1'-(1H-indazol-7-ylcarbonyl)-6-methylspiro[chromene-2,4'-piperidin]-4(3H)-one 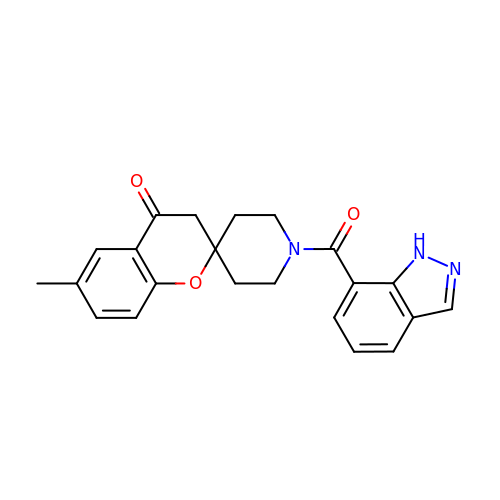| C22 H21 N3 O3 | IKCMGTBANLMNNP-UHFFFAOYSA-N({[6-(4-cyclopropylphenyl)thieno[2,3-d]pyrimidin-4-yl]amino}methanediyl)bis(phosphonic 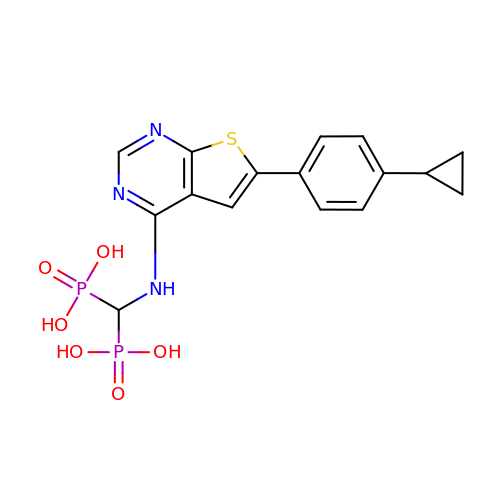acid) | C16 H17 N3 O6 P2 S | VIGDNIIDHDWALF-UHFFFAOYSA-N>MANFPASLLILNGKSADNQPLREAITLLRDEGIQIHVRVTWEKGDAQRYVDEARRLGVETVIAGGGDGTINEVSTALIQIRDGVAPALGLLPLGTANDFATSAGIPEALDKALKLAIAGNAMEIDMAMVNDKTCFINMATGGFGTRITTETPEKLKAALGGVSYLIHGLMRMDTLTPDRCEIRGENFHWQGDALVIGIGNGRQAGGGQQLCPTALINDGLLQLRIFTGEELLPALFSTLTQSDDNPNIIDGASAWFD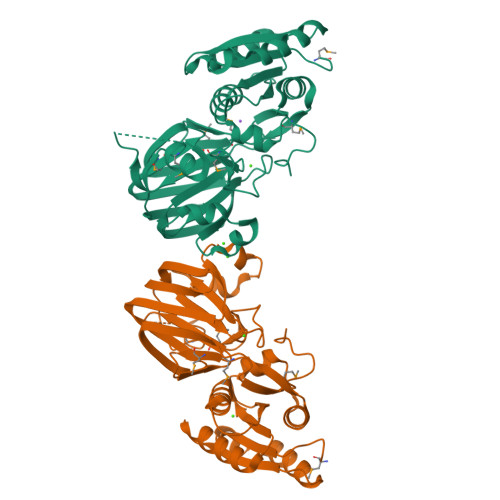IHAPHEITFNLDGEPLSGQEFHIEVLPGALRCRLPPDCPLLR[4x]> ALNVSRLLLPSRVRHSYTGKMGAVFIFVGALTVLFGAIAYGEVTAAAATGDAAAVQEA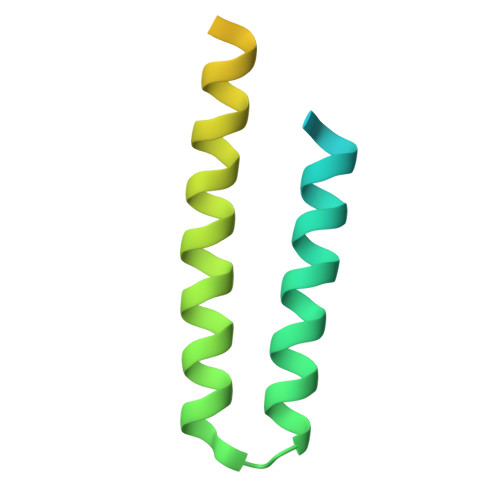AVSAILGLIILLGINLGLVAATLGGDTAASLSTLAAKASRMGDGDLDVELETRRENSHHHHHHH> MSGIPEITAYPLPTAQQLPANLARWSLEPRRAVLLVHDMQRYFLRPLP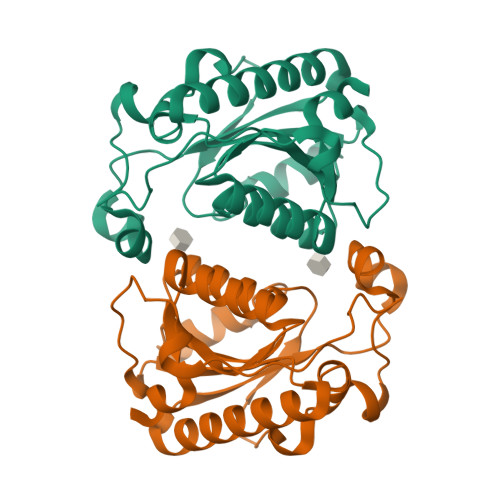ESLRAGLVANAARLRRWCVEQGVQIAYTAQPGSMTEEQRGLLKDFWGPGMRASPADREVVEELAPGPDDWLLTKWRYSAFFHSDLLQRMRAAGRDQLVLCGVYAHVGVLISTVDAYSNDIQPFLVADAIADFSEAHHRMALEYAASRCAMVVTTDEVLE> MTDTQYIGRFAPSPSGELHFGSLIAALGSYLQARARQGRWLVRIEDIDPPREVPGAAETILRQLEHYGLHWDGDVLWQSQRHDAYREALAWLHEQGLSYYCTCTRARIQSIGGIYDGHCRVLHHGPDNAAVRIRQQHPVTQFTDQLRGIIHADEKLAREDFIIHRRDGLFAYNLAVVVDDHFQGVTEIVRGADLIEPTVRQISLYQLFGWKVPDYIH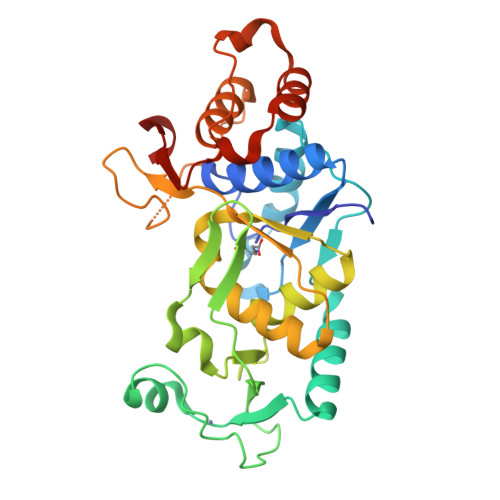LPLALNPQGAKLSKQNHAPALPKGDPRPVLIAALQFLGQQAEAHWQDFSVEQILQSAVKNWRLTAVPESAIVNSTFSNASC(2S)-3-cyclopentyl-N-(5-methylpyridin-2-yl)-2-[2-oxo-4-(trifluoromethyl)pyridin-1(2H)-yl]propanamide 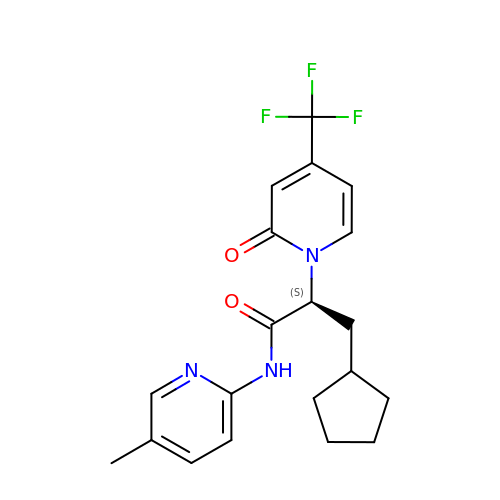| C20 H22 F3 N3 O2 | QRULBTPYHROTAY-INIZCTEOSA-N>MSSSVPTVKLFIGGKFVESKSDKWIDIHNSATNEVIGRVPQATKAEMDAAIASCKRAFPAWADTSVLSRQQVLLRYQQLIKENLKEIAKLITLEQGKTLADAEGDVFRGLQVVEHACSVTSLMMGETMPSITKDMDLYSYRLPLGVCAGIAPFNFPAMIPLWMFPMAM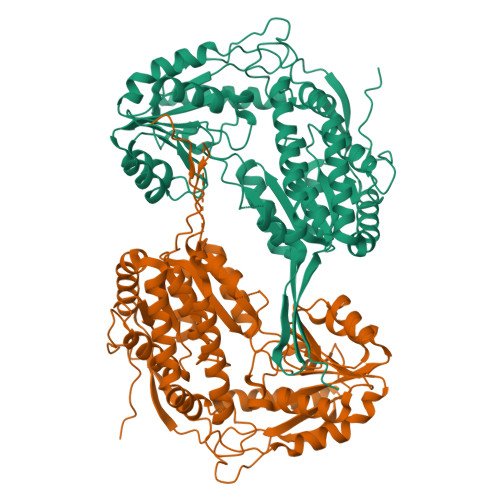VCGNTFLMKPSERVPGATMLLAKLLQDSGAPDGTLNIIHGQHEAVNFICDHPDIKAISFVGSNKAGEYIFERGSRHGKRVQANMGAKNHGVVMPDANKENTLNQLVGAAFGAAGQRCMALSTAVLVGEAKKWLPELVEHAKNLRVNAGDQPGADLGPLITPQAKERVCNLIDSGTKEGASILLDGRKIKVKGYENGNFVGPTIISNVKPNMTCYKEEIFGPVLVVLETETLDEAIQIVNNNPYGNGTAIFTTNGATARKYAHLVDVGQVGVNVPIPVPLPMFSFTGSRSSFRGDTNFYGKQGIQFYTQLKTITSQWKEEDATLSSPAVVMPTMGRENLYFQ[2x]>MGSSHHHHHHSSGLVPRGSHMASYALNNNSDFNNGWKFTLSDSVCYSFVNYNPSSWKTVNLPHDWSVDLPFESTAEGCTGFLKGGIGWYSKTFDTPDNFVDKKCYIVFDGVYNNSEYWINGRKLGFHPYGYSPFFYDISDYLNPKGQENRISVRIDHSRYADSRWYTGSGIYRETQLIFTDKLHIPVWGTFVTTPVVSSERATVNIEVRVKNDYSGPRAGEVRTSYFDSKNKKVGEKLTSFLIEAGKEMKINQSVEISNPSLWDVDSPSMYLAKSEILVDGNVVDTKETPFGIRSIKFDAKKGFFLNGKNMKIKGVCLHHDASMIGAALVEDVWRRRLQTLKDGGCNAIRLSHNPGADAFLELCDEMGFLVQEEFFDEWDYPKDKRLNMDEQSIDYITRGYCEYFQEWAERDLKNVMLRSRNHPCIFQWSIGNEIEWTYKGCKESTGFFSADAGGGYFWNQPPYSTQRIREEWAKQPKQTYDIGRTAKKLAAWTREMDTTRPVTANCILPSISYETGYIDALDVAGFSYRRVMYDYAHKNYPDKPAMGTENLGQWHEWKAVIERDYIPGMFIWTGVDYLGEVGTKGREWPQRAIGCGLLDLAGFEKPSFHMMKSLWTDAPFIAIYSQTANKSSYVEKDGKFTDKDPKKPWTQRLWVWEDVNSHWNYTKGEKVVVEIYSNCDEIELFQNGKSLGKRFLKDFEDHIYKWSVDFKDGNIVAKGKKNGKKTTSAIYTTKETNSIKLSVDKVAVDAN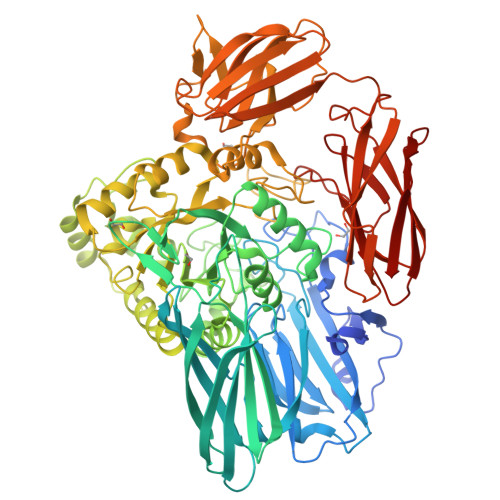NTDVIHVTAQLIDRNGRNISWEEKEITFNIGGNYRLLGVENGDHLNVLNYKSNTVKTYKGRALLVLQATDKAGILNINANSGSISSNDLKVEVK[4x]> GAEFTNPRVRMPEGTTKRVFKGYEEIHVPPPKKRSDPTDQNIPVTELPEWARIPFNTTKTLNKIQSKCFPTAFLDDGNMLVCAPTGSGKTNVAMLTMLREIGKNRNEKGEIDLDAFKIVYIAPLKALVQEQVGNFGKRLEPYGIKVSELTGDRQLTKQQISETQVIVTTPEKWDVITRKATDISYTNLVRLIIIDEIHLLHDDRGPVLESIVSRTIRRTEQTGEPVRIIGLSATLPNYRDVASFLRVDFEKGLFYFDGSYRPCPLRQEFIGVTDKKAIKQLKTMNDITYQKVLEHVGQNRNQMLIFVHSRKETAKTAKYIRDKALEMDTINQILKHDAGTREVLQEAASSVNNTDLKDLLPYGFGIHHAGMSRADRTDVEDLFASGHIQVLVCTATLAWGVNLPAHTVIIKGTQVYSPEKGSWVELSPQDVLQMLGRAGRPQYDTYGEGIIITTQGEIPYYLSLLNQQLPIESQLVSKLVDSLNAEIVLGNVRNRDEGVEWLGYTYLFVRMLRSPGLYSVGAEYEDDVALEQKRVDLIHSAAMVLKKSNLIKYDEKTGKMQATELGRIASHYYISHESMDTYNKLIHPAMNDVELFRVFAQSGEFKYIPVRQEEKLELAKLLARVPIPVKESIEEPTAKINVLLQAYISRLKLEGLALMADMVYVTQSAGRILRAIFEICLKKGWASVAKLALNMCKMAEKRMWPTMSPLRQYPTCPAEIIKKAERMDVP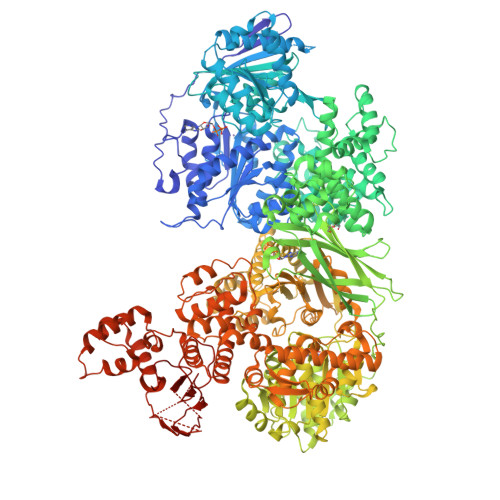WSSYFDLDPPRMGELLGMPKAGKTVCALVSKFPRVEIQGNVQPMTRSMLRIELTITPNFQWDVELHGVTESFWILVEDCDGEEILFHDVFILRKDLAEAEENEHTVEFTVPISEPMPPNYFISVISDRWMHSETRMPVSFQKLILPERFPPHTELLDLQPLPVSALKAKDYAALYPNWQQFNKIQTQTFNSLYNTDNNVLVAAPTGSGKTVCAEFALLRHWAKKDAGRAVYIAPFQELVDLRFQDWQKRLSHLRGGKEIVKLTGETTTDLKLLEQGDLILATPLQWDVLSRQWKRRKNVQTVELFIADDLHMLGGQMGYIYEIVVSRMHFIRTQTELPMRIVGLSVSLANARDIGEWIDAKKHDIYNFSPHVRPVPLELHIQSYTIPHFPSLMLAMAKPTYLAITQLSPDQPAIVFVPSRKQTRATARDLLTACLADDDEDRFLHVEVDQIRKLLDHVQEEALAEALSHGVGYYHEALSQSDKRIVKHLYNNGAIQVLIASRDVCWELDFTAHLVVVMGTQFFEGKEHRYIDYPLSEVLQMFGKALQPSKDGRSRGVLMLPAVKREYYKKFLNEALPVESHLHNFLPDAFVTEISTKMIESGEDAINWATFTYFYRRLLANPSYYGLQDPTHDGLSQYLSDLVETTLKQLSDARIIEMDEDEGTVAPLNAAMIAAYYNISYMTMEMFLLSLSHKSKLRTILEIVTAATEFESIQTRRHEEGILKRIYDHVPVKMNNPVWDSAHFKAFVLVQAHFSRMNLPIDLAKDQEVILQKILSLLSAIVDILSSEGHLNALNAMEMSQMVVQAMWDRDSPLKQIPNFTPEVVKVANKYGINDIFDFMEQMNPEENPNYASLVKDLGLTQAQLAQAANFTNNKYPDITLEFEVDDPDNIRAGEPAYLKIHIERELEEDEEFDPTVHAPFYPGKKSENWWLVVGEESTKTLLAIKRVTVGKELNVKLEFVVPSPGKHDLKLFLMSDSYVGVDQDPSFSVNVAEG>GVQLTAAQELMIQQLVAAQLQCNKRSFSDQPKVTPWPLGADPQSRDARQQRFAHFTELAIISVQEIVDFAKQVPGFLQLGREDQIALLKASTIEIMLLETARRYNHETECITFLKDFTYSKDDFHRAGLQVEFINPIFEFSRAMR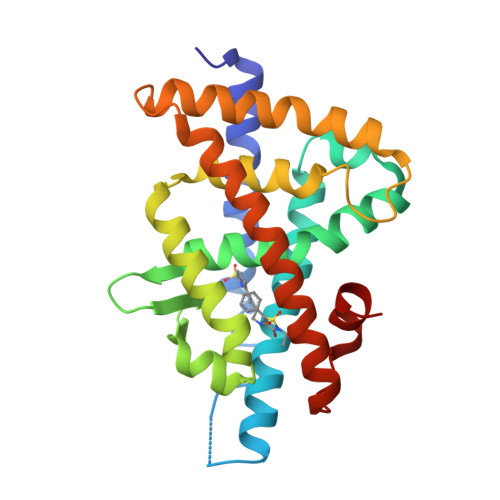RLGLDDAEYALLIAINIFSADRPNVQEPGRVEALQQPYVEALLSYTRIKRPQDQLRFPRMLMKLVSLRTLSSVHSEQVFALRLQDKKLPPLLSEIWDVHE[3x]> GAMESKKRQWALEDFEIGRPLGKGKFGNVYLAREKQSKFILALKVLFKAQLEKAGVEHQLRREVEIQSHLRHPNILRLYGYFHDATRVYLILEYAPRGEVYKEL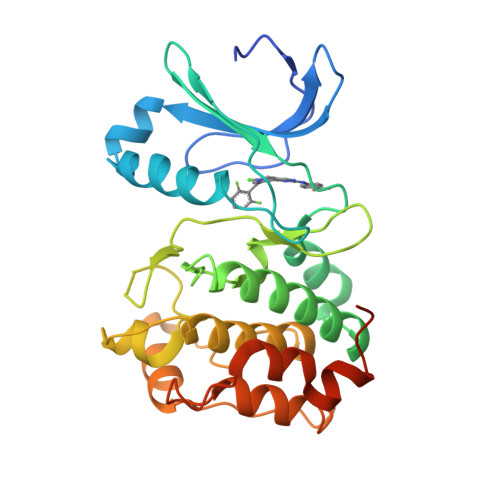QKLSKFDEQRTATYITELANALSYCHSKRVIHRDIKPENLLLGSAGELKIADFGWSVHAPSSRRTTLCGTLDYLPPEMIEGRMHDEKVDLWSLGVLCYEFLVGKPPFEANTYQETYKRISRVEFTFPDFVTEGARDLISRLLKHNPSQRPMLREVLEHPWITANSSKPSNCQNKESASKQS> MSEEKTYKRVEQDDPVPELDIKQGPVRPFIVTDPSAELASLRTMVTLKEKLLVACLAVFTAVIRLHGLAWPDSVVFDEVHFGGFASQYIRGTYFMDVHPPLAKMLYAGVASLGGFQGDFDFENIGDSFPSTTPYVLMRFFSASLGALTVILMYMTLRYSGVRMWVALMSAICFAVENSYVTISRYILLDAPLMFFIAAAVYSFKKYEMYPANSLNAYKSLLATGIALGMASSSKWVGLFTVTWVGLLCIWRLWFMIGDLTKSSKSIFKVAFAKLAFLLGVPFALYLVFFYIHFQSLTLDGDGASFFSPEFRSTLKNNKIPQNVVADVGIGSIISLRHLSTMGGYLHSHSHNYPAGSEQQQSTLYPHMDANNDWLLELYNAPGESLTTFQNLTDGTKVRLFHTVTRCRLHSHDHKPPVSESSDWQKEVSCYGYSGFDGDANDDWVVEIDKKNSAPGVAQERVIALDTKFRLRHAMTGCYLFSHEVKLPAWGFEQQEVTCASSGRHDLTLWYVENNSNPLLPEDTKRISYKPASFISKFIESHKKMWHINKNLVEPHVYESQPTSWPFLLRGISYWGENNRNVYLLGNAIVWWAVTAFIGIFGLIVITELFSWQLGKPILKDSKVVNFHVQVIHYLLGFAVHYAPSFLMQRQMFLHHYLPAYYFGILALGHALDIIVSYVFRSKRQMGYAVVITFLAASVYFFKSFSPIIYGTPWTQELCQKSQWLSGWDYNCNTYFSSLEEYKNQTLTKRESQPAATSTVEEITIEGDGPSYEDLMNEDGKKIFKDTEGNELDPEV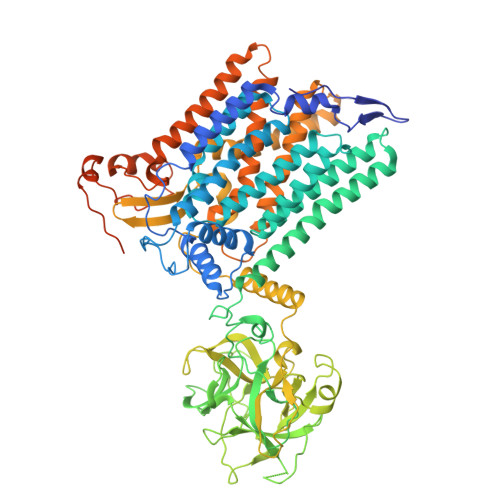VKKMLEEEGANILKVEKRAVLE>[2x]GHMKKPITLEKLVSMVAVGFAETKAETATIKAETATIKKDIAGMKHDIAQLDK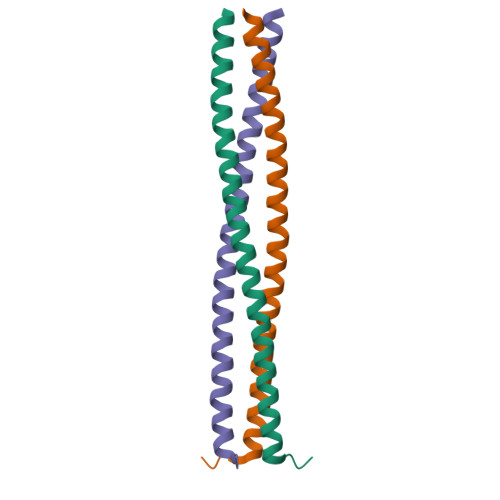RIDGLDKKIADLVDRIGRVESKLDRALNKEVAAWKVSSAS>MSDKDSKNTPQVPEKLGLSRRGFLGASAVTGAAVAATALGGAVMTRESWAQAVKESKQKIHVGPGELDDYYGFWSGGHQGEVRVLGVPSMRELMRIPVFNVDSATGWGLTNESRHIMGDSAKFLNGDCHH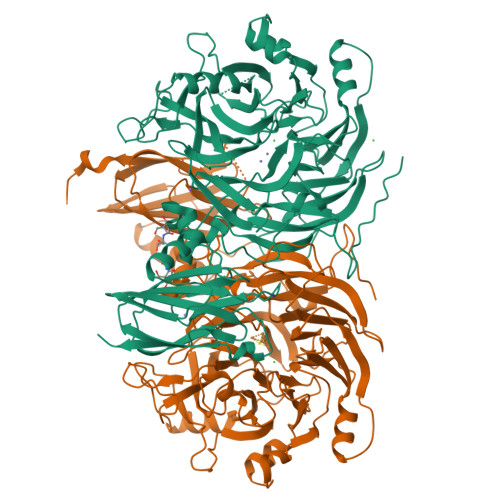PHISMTDGKYDGKYLFINDKANSRVARIRLDIMKCDKMITVPNVQAIHGLRLQKVPHTKYVFANAEFIIPHPNDGKVFDLQDENSYTMYNAIDAETMEMAFQVIVDGNLDNTDADYTGRFAAATCYNSEKAFDLGGMMRNERDWVVVFDIHAVEAAVKAGDFITLGDSKTPVLDGRKKDGKDSKFTRYVPVPKNPHGCNTSSDGKYFIAAGKLSPTCSMIAIDKLPDLFAGKLADPRDVIVGEPELGLGPLHTTFDGRGNAYTTLFIDSQVVKWNMEEAVRAYKGEKVNYIKQKLDVHYQPGHLHASLCETNEADGKWLVALSKFSKDRFLPVGPLHPENDQLIDISGDEMKLVHDGPTFAEPHDCIMARRDQIKTKKIWDRNDPFFAPTVEMAKKDGINLDTDNKVIRDGNKVRVYMTSMAPAFGVQEFTVKQGDEVTVTITNIDQIEDVSAGFVVVNHGVSMEISPQQTSSITFVADKPGLHWYYCSWFCHALHMEMVGRMMVEPAWSHPQFEK[2x]>XTQEYLLKELMKLLKEQIKLLKEQI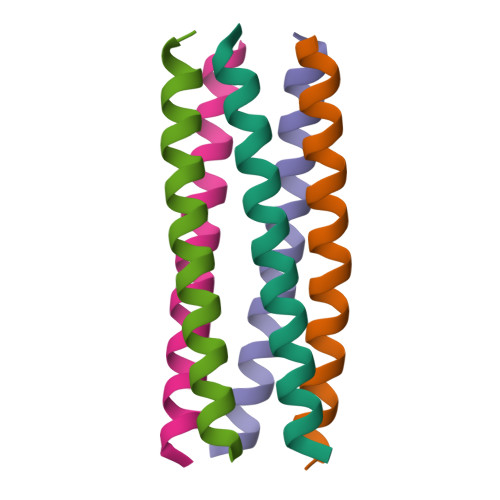KMLKELEKQX[5x]> DLEVANQTLKDEY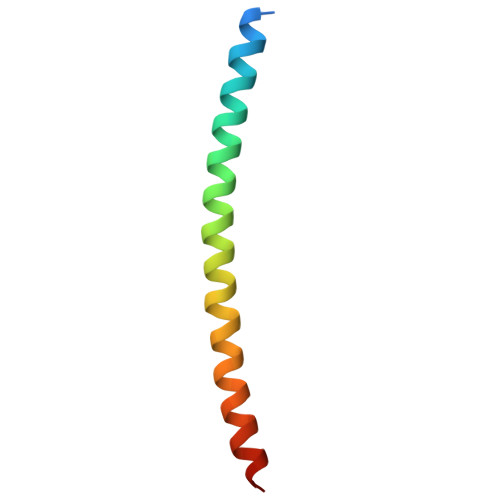DALQITFTALEEKLRKTTEENQELVTRWMAEKAQEANRLNAENE> GAMKITTWNVNSLNVRLPQVQNLLADNPPDILVLQELKLDQDKFPAAALQMMGWHCVWSGQKTYNGVAIVSRSVPQDVHFGLPALPDDPQRRVIAATVSGVRVINVYCVNGEALDSPKFKYKEQWFAALTEFVRDEMTRHGKLVLL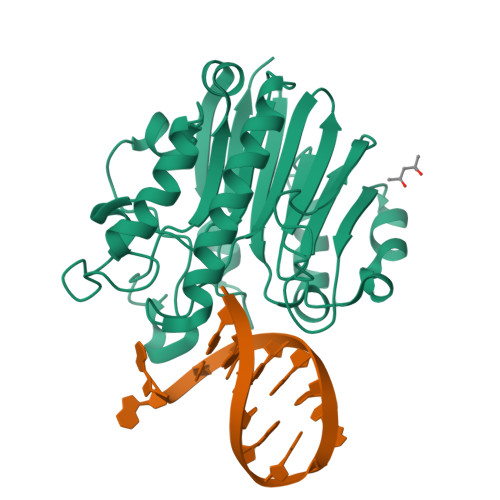GDFNIAPADADCYDPEKWHEKIHCSSVERQWFQNLLDLGLTDSLRQVHPEGAFYTWFDYRGAMFQRKLGLRIDHILVSPAMAAALKDVRVDLETRALERPSDHAPVTAEFDW> GIVKQDSLVINLNRSNPKLKDLYIRPNIAQKRMQGSLEAHVNGFRFTSVRGDKVDILYNNIKHALFQPCDGEMIIVLHFHLKNAIMFGKKRHTDVQFYTEVGEITTDLGKHQHMHDRDDLYAEQMEREMRHKLKTAFKNFIEKVEALTKEELEFEVPFRDLGFNGAPYRSTCLLQPTSSALVNATEWPPFVV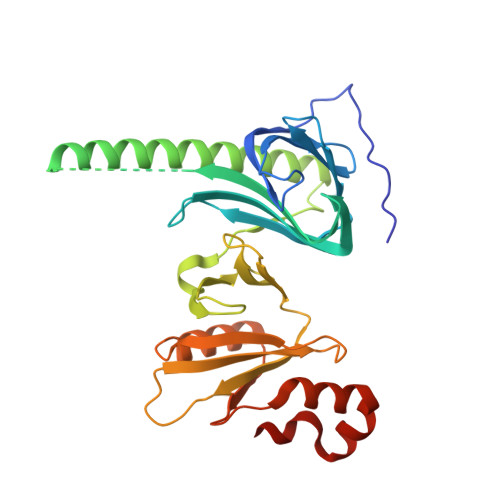TLDEVELIHFERVQFHLKNFDMVIVYKDYSKKVTMINAIPVASLDPIKEWLNSCDLKYTEGVQSLNWTKIMKTIVDDPEGFFEQGGWSFLEPEGE>[4x]MPEAPKKESLEVFDLTLDQKNKQKLQLIEELTSNADQVQRQVLEEILTRNADVEYLRRHDLNGRTDRETFKNIMPVITYEDIEPEINRIANGDKSPILSSKPISEFLTSSGTSGGERKLMPTIEEELDRRSLLYSLLMPVMSQFVPGLENGKGMYFLFIKSESKTPGGLPARPVLTSYYKSSHFKERPYDPYTNYTSPNETILCSDSYQSMYSQMLCGLCQHQEVLRVGAVFASGFIRAIKFLEKHWIELVRDIRTGTLSSLITDPSVREAVAKILKPSPKLADFVEFECKKSSWQGIITRLWPNTKYVDVIVTGTMSQYIPTLDYYSNGLPLVCTMYASSECYFGVNLRPLCKPSEVSYTLIPSMAYFEFLPVHRNNGVTNSINLPKALTEKEQQELVDLV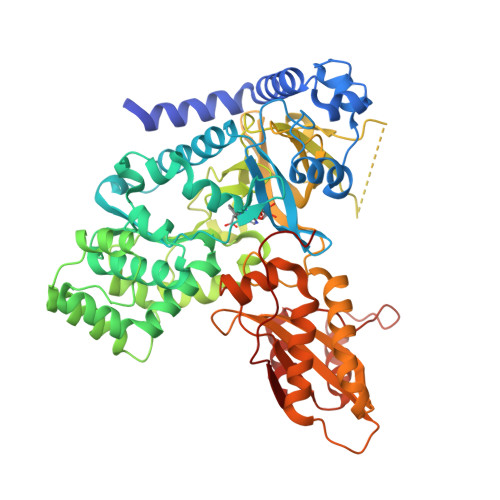DVKLGQEYELVVTTYAGLCRYRVGDLLRVTGFKNKAPQFSFICRKNVVLSIDSDKTDEVELQNAVKNAVTHLVPFDASLSEYTSYADTSSIPGHYVLFWELCLDGNTPIPPSVFEDCCLAVEESFNTVYRQGRVSDKSIGPLEIKIVEPGTFDKLMDYAISLGASINQYKTPRCVKFAPIIELLNSRVVDSYFSPKCPKWVPGHKQWGSN> MAGFLKLLRLLLRRQRLARAMDSFPGPPTHWLFGHALEIQKTGSLDKVVTWTQQFPYAHPLWVGQFIGFLNIYEPDYAKAVYSRGDPKAPDVYDFFLQWIGKGLLVLDGPKWFQHRKLLTPGFHYDVLKPYVAIFADSTRIMLEKWEKKACEGKSFDIFSDVGHMALDTLMKCTFGKGDSGLNHRDSSYYVAVSELTLLMQQRIDSFQYHNDFIYWLTPHGRRFLRACRAAHDHTDRVIRQRKAALQDEKEREKIQNRRHLDFLDILLDVRGESGVQLSDTDLRAEVDTFMFAGHDTTTSGISWFLYCMALYPEHQQRCREEVREILGDQDSFQWEDLAKMTYLTMCMKECFRLYPPVPQVYRQLSKPVSFVDGRSLPAGS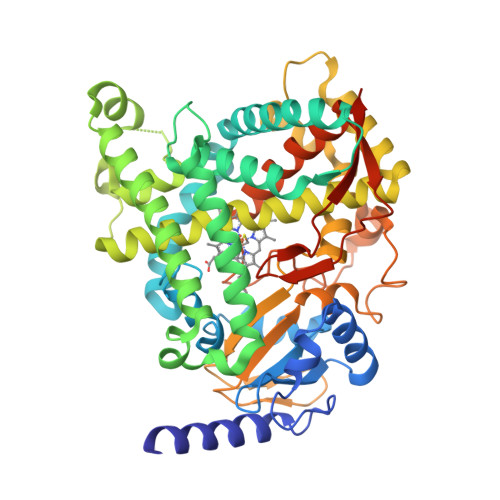LISLHIYALHRNSDVWPDPEVFDPLRFSPENSSGRHPYAFIPFSAGPRNCIGQQFAMNEMKVVTALCLLRFEFSVDPLRLPIKLPQLVLRSKNGIHLYLKPLGPKAEKSTHHHHHH>CGRFAQSQTREDYLALLAEDIERDIPYDPEPIGRYNVAPGTKVLLLSERDEHLHLDPVFWGYAPGWWDKPPLINARVETAATSRMFKPLWQHGRAICFADGWFEWKKEGDKKQPFFIYRADGQPIFMAAIGSTPFERGDEAEGFLIVTAAADQG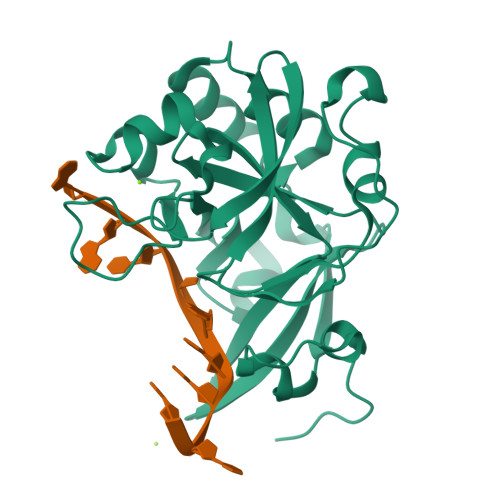LVDIHDRRPLVLSPEAAREWMRQEISGKEASEIAASGCVPANQFSWHPVSRAVGNVKNQGAELIQPVLEVLFQ[4x]> INQVRPKLPLLKILHAAGAQGEMFTVKEVMHYLGQYIMVKQLYDAAAQHMVYCGGDLLGELLGRQSFSVKDPSPLY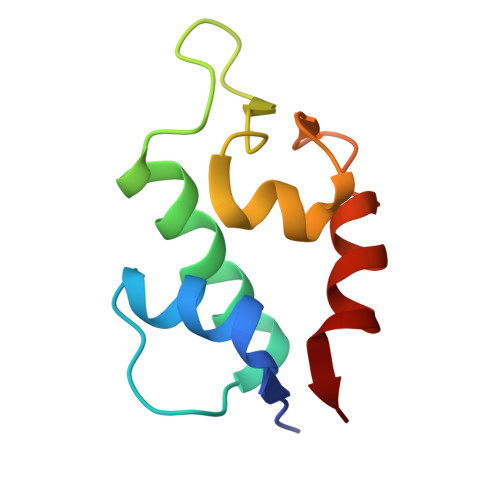DMLRKNLVT> GRSESQMDITDINAP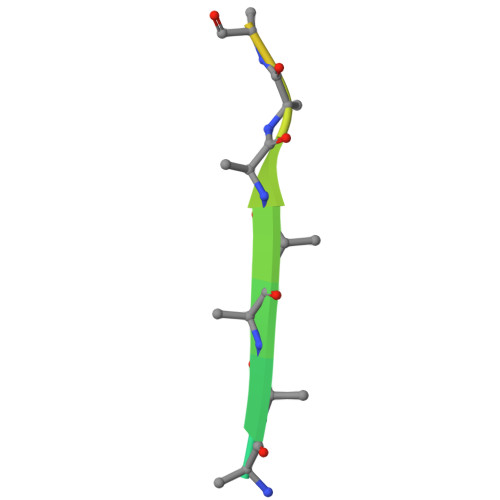KPKKKQR>[2x]MAQGLYVGGFVDVVSCPKLEQELYLDPDQVTDYLPVTEPLPITIEHLPETEVGWTLGLFQ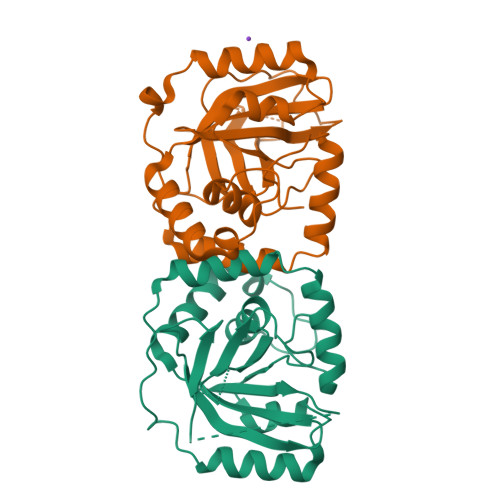VSHGIFCTGAITSPAFLELASRLADTSHVARAPVKNLPKEPLLEILHTWLPGLSLSSIHPRELSQTPSGPVFQHVSLCALGRRRGTVAVYGHDAEWVVSRFSSVSKSERAHILQHVSSCRLEDLSTPNFVSPLETLMAKAIDAGFIRDRLDLLKTDRGVASILSPVYLKA>GPEINKELNQVMEQLGDARIDRQESSRQQRKAEIMESIKRLYPGSVYGRLIDLCQPTQKKYQIAVTKVLGKNMDAIIVDSEKTGRDCIQYIKEQRGEPETFLPLDYLEVKPTDEKLRELKGAKLVIDVIRYEPPHIKKALQYACGNALVCDNVEDARRIAFGGHQRHKTVALDGTLFQKSGVISGGASDLKAKARRWDEKAVDKLKEKKERLTEELKEQMKAKRKEAELRQVQ[6x];>GPLGSGRPQSERNYLWREENAEQQALAAKREDLEKKQQLLRAATGKAILNGIDS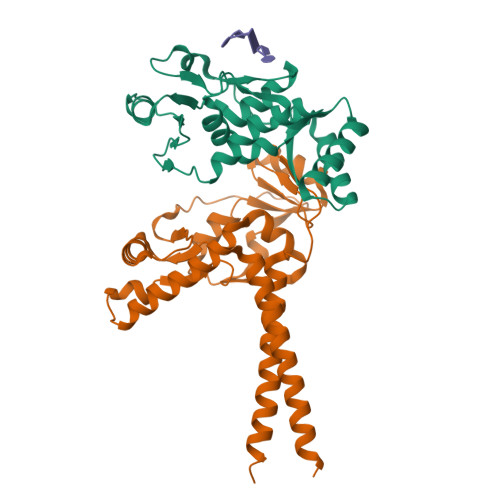INKVLDHFRRKGINQHVQNGYHGIVMNNFECEPAFYTCVEVTAGNRLFYHIVDSDEVSTKILMEFNKMNLPGEVTFLPLNKLDVRDTAYPETNDAIPMISKLRYNPRFDKAFKHVFGKTLICRSMEVSTQLARAFTMDCITLEGDQVSHRGALTGGYYDTRKSRLELQKDVRKAEEELGELEAKLNENLRRNIERINNEIDQ[6x]>[3x]MEGNTILKIVLICTILAGLFGQVVPVYAENTTYQTPTGIYYEVRGDTIYMINVTSGEETPIHLFGVNWFGFETPNHVVHGLWKRNWEDMLLQIKSLGFNAIRLPFCTESVKPGTQPIGIDYSKNPDLRGLDSLQIMEKIIKKAGDLGIFVLLDYHRIGCTHIEPLWYTEDFSEEDFINT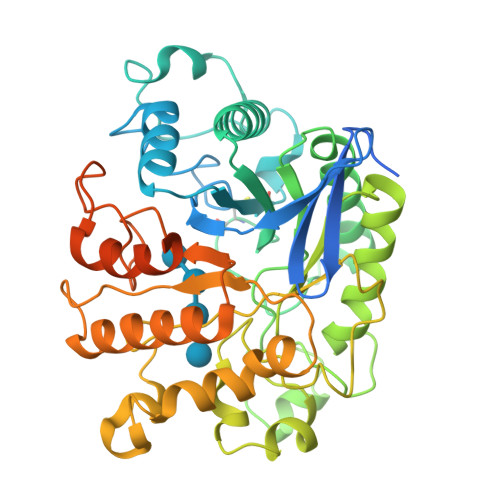WIEVAKRFGKYWNVIGADLKNAPHSVTSPPAAYTDGTGATWGMGNPATDWNLAAERIGKAILKVAPHWLIFVEGTQFTNPKTDSSYKWGYNAWWGGNLMAVKDYPVNLPRNKLVYSPHVYGPDVYNQPYFGPAKGFPDNLPDIWYHHFGYVKLELGYSVVIGEFGGKYGHGGDPRDVIWQNKLVDWMIENKFCDFFYWSWNPDSGDTGGILQDDWTTIWEDKYNNLKRLMDSCSKSSSSTQSVIRSTTPTKSNTSKKICGPAILIILAVFSLLLRRAPR>[4x]MSKEVSEEAQAHQHGKDYVDPPPAPFFDLGELKLWSFWRAAIAEFIATLLFLYITVATVIGHSKETVVCGSVGLLGIAWAFGGMIFVLVYCTAGISGGHINPAVTFGLFLARKVSLLRALVYMIAQCLGAICGVGLVKAFMKGPYNQFGGGANSVALGYNKGTALGAEIIGTFVLVYTVFSATDPKRSARDSHVPILAPLPIGFAVFMVHLATIPITG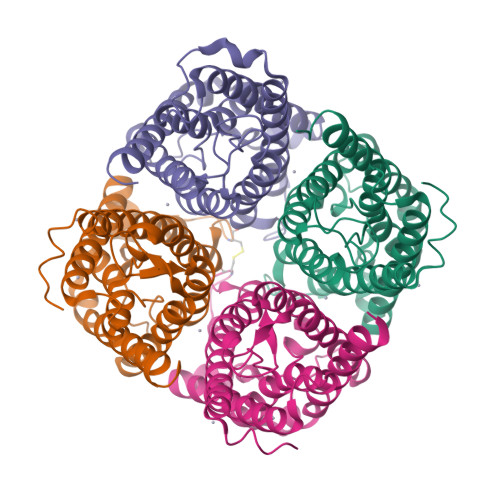TGINPARSFGAAVIFNSNKVWDDQWIFWVGPFIGAAVAAAYHQYVLRAAAIKALGSFRSNPTN>[2x]MKPTVIITGASSGVGLYGAKALIDKGWHVIMACRNLDKTQKVADELGFPKDSYTIIKLDLGYLDSVRRFVAQFRELGRPLKALVCNAAVYFPLLDEPLWSADDYELSVATNHLGHFLLCNLLLEDLKACPDADKRLIILGTVTANS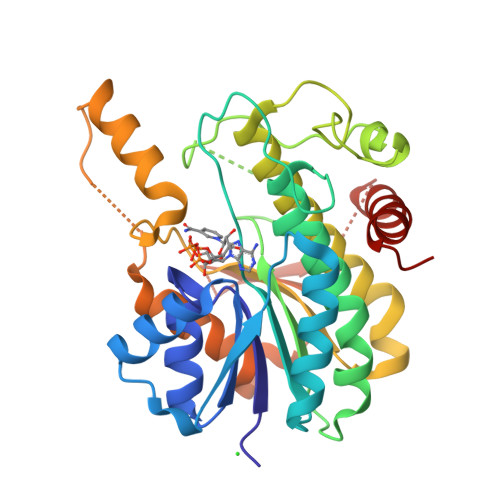KELGGKIPIPAPPDLGNFEGFEAGFKKPIAMINNKKFKSGKAYKDSKLCNMLTTRELHRRFHQETGIVFNSLYPGCVADTPLFRNHYSLFRTIFPWFQKNVTKGYVSQELAGERVAMVVADDKFKDSGVHWSWGNRQQAGREAFVQELSEQGSDAQKAQRMWDLSEKLVGLV>MPLNRTLSMSSLPGLEDWEDEFDLENAVLFEVAWEVANKVGGIYTVLQTKAKVTGDEWGDNYFLVGPYTEQGVRTQVELLEAPTPALKRTLDSMNSKGCKVYFGRWLIEGGPLVVLLDVGASAWALERWKGELWDTCNIGVPWYDREANDAVLFGFLTTWFLGEFLAQSEEKPHVVAHFHEWLAGVGLCLCRARRLPVATIFTTHATLLGRYLCAGAVDFYNNLENFNVDKEAGERQIYHRYCMERAAAHCAHVFTTVSQITAIEAQHLLKRKPDIVTPNGLNVKKFSAMHEFQNLHAQSKARIQEFVRGHFYGHLDFNLDKTLYFFIAGRYEFSNKGADVFLEALARLNYLLRVNGSEQTVVAFFIMPARTNNFNVETLKGQAVRKQLWDTANTVKEKFGRKLYESLLVGSLPDMNKMLDKEDFTMMKRAIFATQRQSFPPVCTHNMLDDSSDPILTTIRRIGLFNSSADRVKV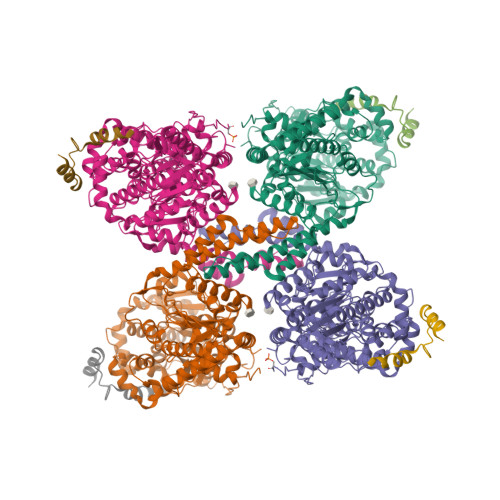IFHPEFLSSTSPLLPVDYEEFVRGCHLGVFPSYYEPWGYTPAECTVMGIPSISTNLSGFGCFMEEHIADPSAYGIYILDRRFRSLDDSCSQLTSFLYSFCQQSRRQRIIQRNRTERLSDLLDWKYLGRYYMSARHMALSKAFPEHFTYEPNEADAAQGYRYPRPASVPPSPSLSRHSSPHQSEDEEDPRNGPLEEDGERYDEDEEAAKDRRNIRAPEWPRRASCTSSTSGSKRNSVDTATSSSLSTPSEPLSPTSSLGEERN[4x];>MTDQAFVTLTTNDAYAKGALVLGSSLKQHRTTRRLVVLATPQVSDSMRKVLETVFDEVIMVDVLDSGDSAHLTLMKRPELGVTLTKLHCWSLTQYSKCVFMDADTLVLANIDDLFDREELSAAPDPGWPDCFNSGVFVYQPSVETYNQLLHLASEQGSFDGGDQGILNTFFSSWATTDIRKHLPFIYNLSSISIYSYLPAFKVFGASAKVVHFLGRVKPWNYTYDPKTKSVKSEAHDPNMTHPEFLILWWNIFTTNVLPLLQQFGLVKDTCSYVNVLSDLVYTLAFSCGFCRKEDVSGAISHLSLGEIPAMAQPFVSSEERKERWEQGQADYMGADSFDNIKRKLDTYLQ[4x]Enteropathogenic *E. coli* (EPEC) O127:H6 encodes an additional, tripartite TA module, *hipBST*, for which the HipT toxin was shown to specifically target tryptophanyl-tRNA synthetase, TrpS. Surprisingly, the function as antitoxin has been taken over by the third protein, HipS, but the molecular details of how activity of HipT is controlled remain poorly understood. Here, we show that HipBST is markedly different from HipBA and that the unique HipS protein, which is homologous to the N-terminal subdomain of HipA, has evolved to function as antitoxin by breaking the kinase active site. We also show how auto-phosphorylation at two conserved sites in the kinase toxin serve to dually regulate binding of HipS and kinase activity.

To understand the individual roles of the two autophosphorylation positions, we next determined crystal structures of two HipBST complexes with HipT serine residues mutated to alanine individually: HipBST^S57A^ (2.4 Å, [Table tblS1]) and HipBST^S59A^ (3.4 Å). The phosphate groups on Ser57 (in S59A) and Ser59 (in S57A) are shown in orange and relevant nearby residues are highlighted. **b.** Close-up of the HipT active site as observed for the S57A mutant with relevant active site residues shown as sticks. In both structures, however, the Gly-rich loop maintains its outward conformation, incompatible with ATP binding, suggesting that HipT is inactive. The phosphate group on Ser59 occupies a position very similar to phosphorylated Ser150 in HipA_Ec_, despite the fact that this residue aligns to Ser57 at the sequence level ([Fig figS4], **top and 1b**). This position structurally overlaps with the γ phosphate of ATP in the structure of ATP-bound HipA_Ec_, suggesting that phosphorylation prevents nucleotide binding in the kinase active site ([Fig fig4]). Here, we observed a marked difference in migration between HipT from wildtype HipBST, HipBST^S59A^, and HipBST^S57A^ confirming that HipT^S57A^ is predominantly phosphorylated while HipT^S59A^ is only partially modified, consistent with the crystal structures. In summary, we conclude that the conformation of the HipT active site loop (Gly-rich loop) inside the HipBST complex is independent of the autophosphorylation state. We still don’t understand what controls whether HipT becomes modified at one or the other position but the structures of HipT^S57A^ and HipT^S59A^ could suggest that subtle changes in the loop can make a big difference ([Fig fig4]). Free HipT could then form three populations, non-phosphorylated HipT, HipT P-Ser57, and HipT P-Ser59. Furthermore, HipT P-Ser59 would readily be able to (re-)bind HipS, and therefore form a stable and inactive HipBST complex as well as tightly bind the *hipBST* promoter, effectively shutting down the kinase activity, halting the expression of new protein.

>MICSGPQNLAQELKAIGDQLQELQKKLIQGPNISQPRPLLTIETPRHLGEQLNARRKELGIDLYTLELQTGISTSTLKRLFKDPEQVKFGSVFAVANVLGVKLCIGE[2x];>[2x]MHRRVKVLLYGQVVGELSQNDSGFLFQYAHDYHGPAISISLPVAQRQFPSETLHPYFASLAPEGWLRQRYSQIQHRDENDLLGMLIDNGKNLLGAIQILPWEE;>[2x]MANCRILLTPLNERDEQRGYSTQGLKRLSGTAKLNPRLGFTRTQFVQELPRQQKGMAISGYQPKLQLVLDEGEFRVVDHQGNFILKPSPADFPGLAENEHATMTLMSRLGFDVPVHGLLSFAPQSEEELEYAFVIRRYDRDNKGLPVHQEQLDGAMQITDKYGKTGNDNEQYVSYETLARFLVAHVNDNIAFKIDLFRRIVYAWLLGNNDMHLRNFGLVYSDGLTPALAPVYDFVSVAPYPEYFYSNYLALPLLTREEGGRELAPGFHSDYGEYIGQDFLLLGESMGLAPRLLEKLFQDIRKENAIVMETYEQSFMTQDHIQAVLQCYRHRLGLLHHHHHH> ADKELKFLVVDDFSTMRRIVRNLLKELGFNNVEEAEDGVDALNKLQAGGFGFIISDWNMPNMDGLELLKTIRADSAMSALPVLMVTAEAK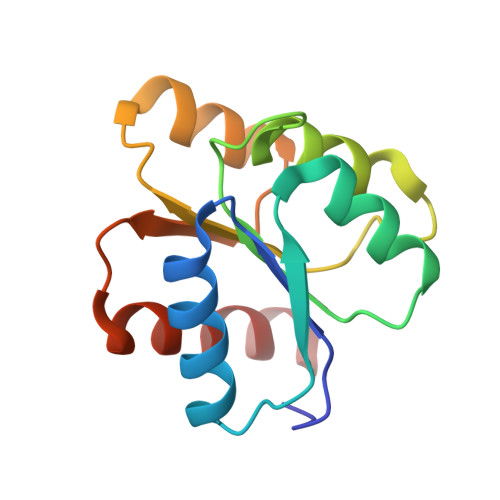KENIIAAAQAGASGYVVKPFTAATLEEKLNKIFEKLGM>[4x]MYAIAFDLVVKDTQDYH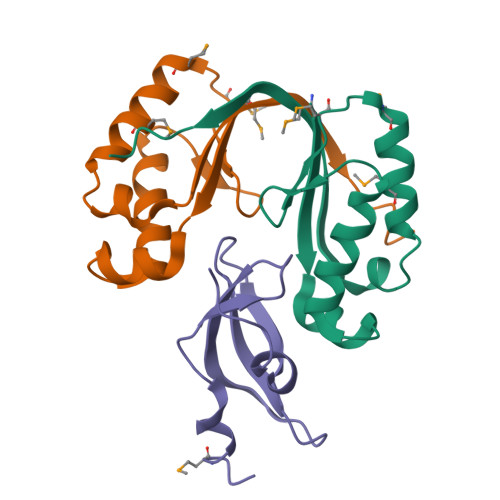PKGVQEAYTDIGAVLAKFGFVRTQGSLYTNMNEDMANLFQAMNALKQLAWISQSVRDIRAFRIEQWSDFTDFIRNLEHHHHHH;>MASMTGGQQMGRDPNSSSMELRQQIPTGCIKQFGQFGVPYVVGEVAEFLPDGDVLVNITLLQSGEKDIYRLSYLLEDPEAE[2x]> MENTENSVDSKSIKNLEPKIIHGSESMDSGISLDNSYKMDYPEMGLCIIINNKNFHKSTGMTSRSGTDVDAANLRETFRNLKYEVRNKNDLTREEIVELMRDVSKEDHSKRSSFVCVLLSHGEEGIIFGTNGPVDLKKIVNFFRGDRCRSLTGKPKLFIIQACRGTELDCGIETDSGVDDDMACHKIPVEADFLYAYSTAPGYYSWRNSKDGSWFIQSLCAMLKQYADKL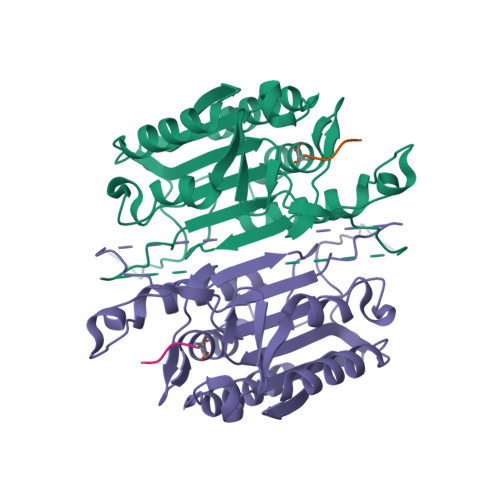EFMHILTRVNRKVATEFESFSFDATFHAKKQIPCIVSMLTKELYFYHL>MRSRRVDVMDVMNRLILAMDLMNRDDALRVTGEVREYIDTVKIGYPLVLSEGMDIIAEFRKRFGCRIIADFKVADIPETNEKICRATFKAGADAIIVHGFPGADSVRACLNVAEEMGREVFLLTEMSQPGAEMFIQGAADE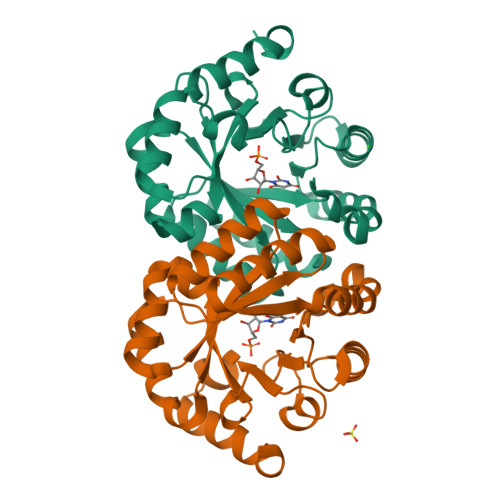IARMGVDLGVKNYVGPSTRPERLSRLREIIGQDSFLISPGVGAQGGDPGETLRFADAIIVGRSIYLADNPAAAAAGIIESIKDLLNP[2x]> GAMSEQLEQMASIVSATRYLKMRCNRSDLPDEQSILNVANRIAIGKGWQSLTQEDIRKHSDD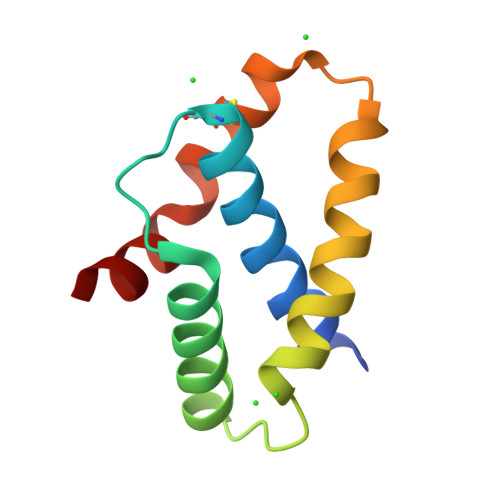IYVRLTRDSTPEYIKCREFNRRLVPFIGELLA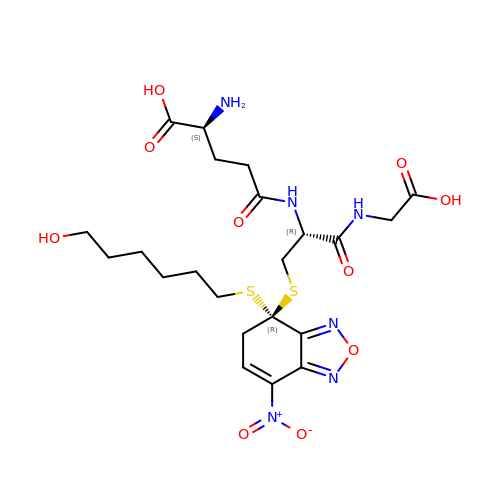L-gamma-glutamyl-S-{(4R)-4-[(6-hydroxyhexyl)sulfanyl]-7-nitro-4,5-dihydro-2,1,3-benzoxadiazol-4-yl}-L-cysteinylglycine | C22 H32 N6 O10 S2 | DZIARIAPFJPVSN-FBJOKTGGSA-N> MTSRKKVLLKVIILGDSGVGKTSLMNQYVNKKFSNQYKATIGADFLTKEVMVDDRLVTMQIWDTAGQERFQSLGVAFYRGADCCVLVFDVTAPNTF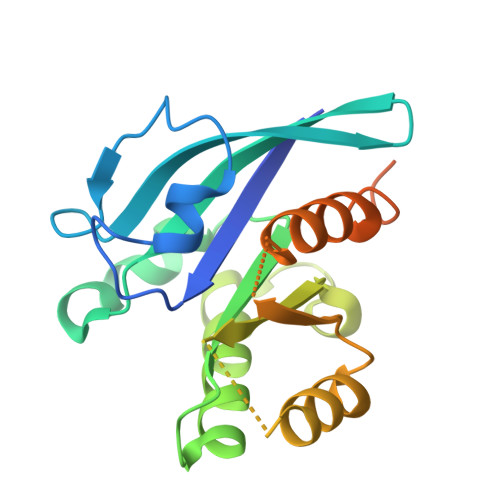KTLDSWRDEFLIQASPRDPENFPFVVLGIKIDLENRQVATKRAQAWCYSKNNIPYFETSAKEAINVEQAFQTIARNALKQETEVELYNEFPEPIKLDKNDRAKASAESCSC>[2x]GELVRTDSPNFLCSVLPTHWRCNKTLPIAFKVVAKGDVPDGTLVTVMAGNDENYSAELRNATAAMKNQVARFNDLRFVGRSGRGKSFTLTITVFTNPPQVATYHRAIKITVDGPREPRRHRQKLDDQTKPGSLSFSERLSELEQLRRTAMRVSPHHPAPTPNPRASLNHSTAFNPQPQSQMQDARQIQPSPPWSYDQSYQYLGS;>[2x]MPRVVPDQRSKFENEEFFRKLSRECEIKYTGFRDRPHEER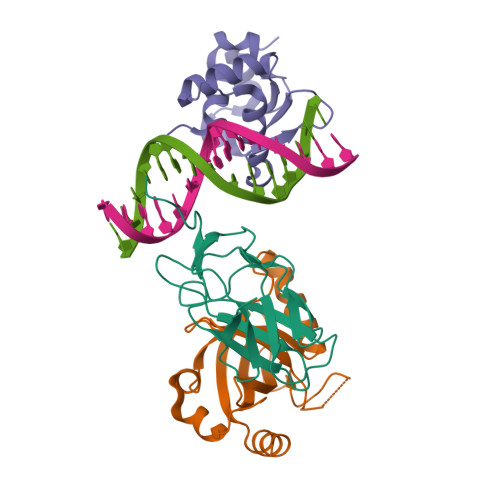QTRFQNACRDGRSEIAFVATGTNLSLQFFPASWQGEQRQTPSREYVDLEREAGKVYLKAPMILNGVCVIWKGWIDLHRLDGMGCLEFDEERAQQEDALAQQA;>[2x]SLQRVPSYDSFDSEDYPAALPNHKPKGTFKDYVRDRADLNKDKPVIPAAALAGATGSGPIQLWQFLLELLTDKSCQSFISWTGDGWEFKLSDPDEVARRWGKRKNKPKMNYEKLSRGLRYYYDKNIIHKTAGKRYVYRFVCDLQSLLGYTPEELHAMLDVKPDADE>[8x]QECDFTPMLTGTPPPIYNFKRLVFTNCNY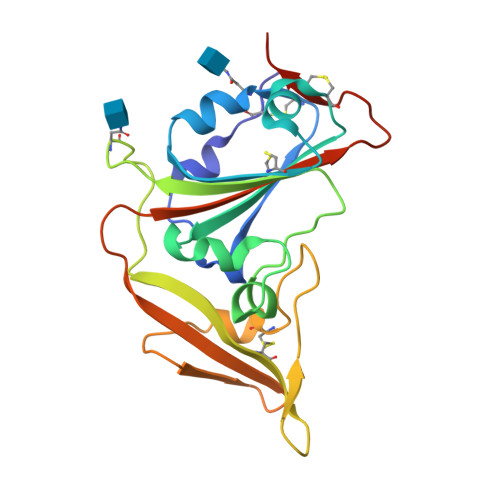NLTKLLSLFQVSEFSCHQVSPSSLATGCYSSLTVDYFAYSTDMSSYLQPGSAGAIVQFNYKQDFSNPTCRVLATVPQNLTTITKPSNYAYLTECYKTSAYGKNYLYNAPGAYTPCLSLASRGFSTKYQSHSDGELTTTGYIYPVTGNLQMAFIISVQYGTDTNSVCPMQHHHHHH>MERPQPDSMPQDLSEALKEATKEVHTQAENAEFMRNFQKGQVTRDGFKLVMASLYHIYVALEEEIERNKESPVFAPVYFPEELHRKAALEQDLAFWYGPRWQEVIPYTPAMQRYVKRLHEVGRTEPELLVAHAYTRYLGALSGGQVLKKIAQKALDLPSSGEGLAFFTFPNIASATKFKQLYRSRMNSLEMTPAVRQRVIE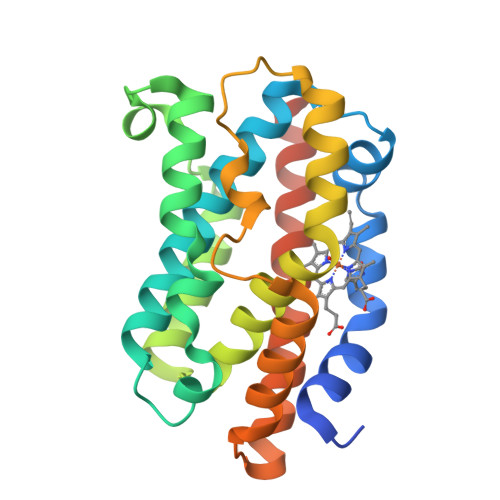EAKTAFLLNIQLFEELQELLTHDTKDQSPSRA[2x]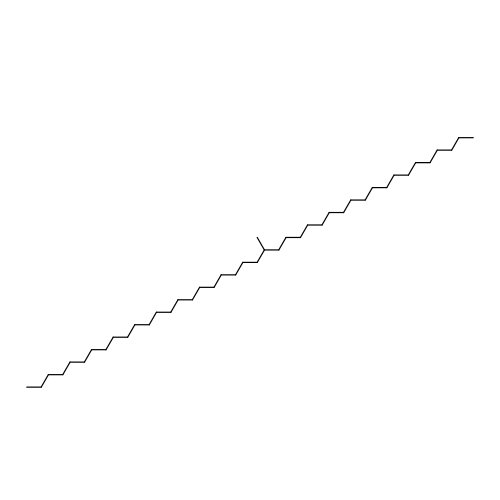(20S)-20-methyldotetracontane | C43 H88 | RQRQHJNVHOWJHC-QLKFWGTOSA-N>[4x]MIPDVSQALAWLEKHPQALKGIQRGLERETLRVNADGTLATTGHPEALGSALTHKWITTDFAEALLEFITPVDGDIEHMLTFMRDLHRYTARNMGDERMWPLSMPSYIAEGQDIELAQYGTSNTGRFKTLYREGLKNRYGALMQTISGVHYNFSLPMAFWQAKSGDISGADAKEKISAGYFRVIRNYYRFGWVIPYLFGASPAISSSFLQGKPTSLPFEKTESGMYYLPYATSLRLSDLGYTNK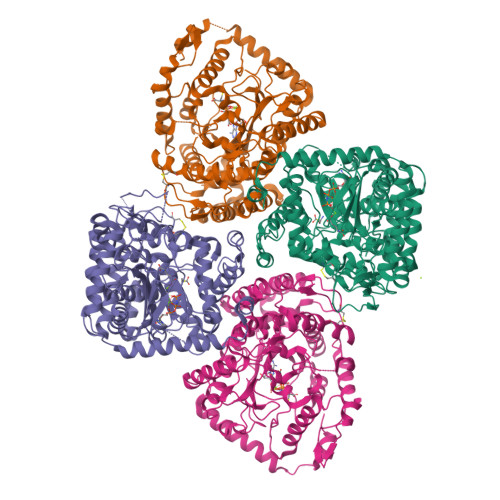SQSNLGITFNDLYEYVAGLKQAIKTPSEEYAKIGIEKDGKRLQINSNVLQIENELYAPIRPKRVTRSGESPSDALLRGGIEYIEVRSLDINPFSPIGVDEQQVRFLDLFMVWCALADAPEMSSSELACTRVNWNRVILEGRKPGLTLGIGCETAQFPLPQVGKDLFRDLKRVAQTLDSINGGEAYQKVCDELVACFDNPDLTFSARILRSMIDTGIGGTGKAFAEAYRNLLREEPLEILREEDFVAEREASERRQQEMEAADTEPFAVWLEKHA> IPCGESCVWLPCISSAIGCSCKSK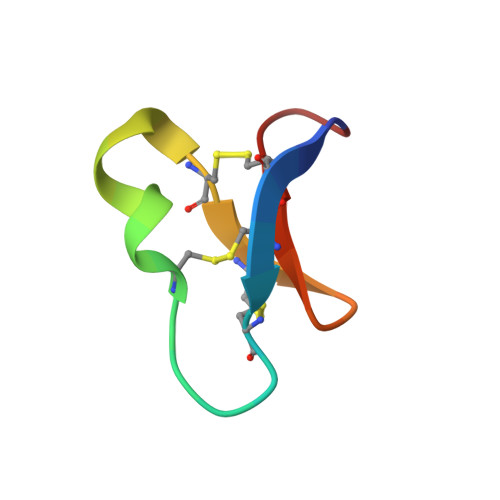VCYRNG> GLFDAPGRSQFVPADQAFAFDFQQNQHDLNLTWQIKDGYYLYR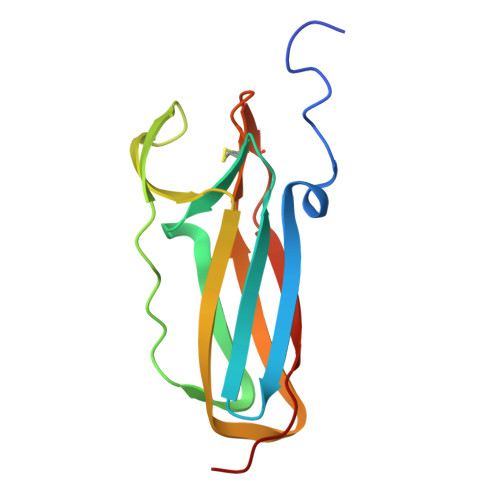KQIRITPEHAKIADVQLPQGVWHEDEFYGKSEIYRDRLTLPVTINQASAGATLTVTYQGCADAGFCYPPETKTVPLSEVVAN>HHMSSKQFKILVNEDYQVNVPSLPIRDVLQEIKYCYRNGFEGYVFVPEYCRDLVDCDRKDHYVIGVLGNGVSDL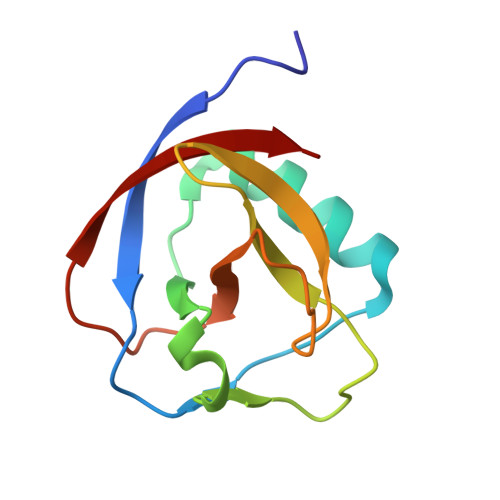KPVLLTEPSVMLQGFIVRSGSGSVLEDFDLKIA[2x]> GPGSAEKKVEAKVEVAENNVSSVARREKELYDQIAD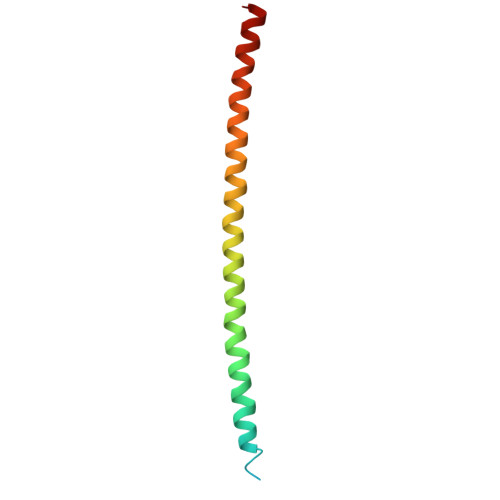LTDKNGEYLERIGELEERQKNLEKLEHQSQVAADKHYQEQAKKHQEYKQEQEER> MGAKYKKEFAAYTAALAEAESKKKQDGYLSEPRSQSLNFKSEPNAIRTIDSSVHQYGQQELDALVKSWGISPTNPDRKKSTAYSYFNAINSNNTYAKLVLEKDKPVDVTYTGLKNSSFNGKKISKVVYTYTLKETGFNDGTKMTMFASSDPTVTAWYNDYFTSTNINVKVKFYDEEGQLMNLTGGLVNFSSLNRGNGSGAIDKDAIESVRNFNGRYIP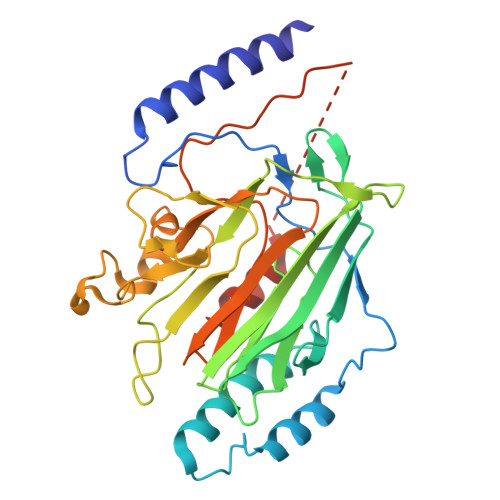ISGSSIKIHENNSAYADSSNAEKSLGARWNTSEWDTTSSPNNWYGAIVGEITQSEISFNMASSKSGNIWFAFNSNINAIGVPTKPVAPTAPTQPMYETEKPLENLYFQGAAALEHHHHHH While most SAM riboswitches strongly discriminate between SAM and SAH, the SAM/SAH riboswitch responds to both ligands with similar apparent affinities. The riboswitch forms an H-type pseudoknot structure with coaxial alignment of the stem–loop helix (P1) and the pseudoknot helix (PK). An additional three base pairs form at the non-open end of P1, and the ligand is bound at the interface between the P1 extension and the PK helix. Binding SAM or SAH stabilizes the PK helix, so structuring the Shine–Dalgarno sequence, sequestering it and preventing initiation of translation (OFF state).

The SAH ligand is located at the interface between the P1 and PK helices. The adenine moiety adopts an anti conformation, and the nucleobase is stacked between G46 and G24. It forms a trans Hoogsteen-Watson Crick base pair with U23 thus becoming an integral part of the coaxial P1-PK helices. The homocysteine chain is directed into the major groove of the P1 helix. The SAH adenine:U23 base pair is connected by two hydrogen bonds, i.e. adenine N6 to U23 O2 (2.9 Å) and U23 N3 to adenine N7 (2.7 Å). In addition, SAH adenine N1 accepts a hydrogen bond from U44 O2′ (2.7 Å), and the SAH O2′ donates one to G46 N7 (2.7 Å). Lastly the SAH methionyl amide N donates a hydrogen bond to U23 O4 (2.8 Å). Thus, altogether the SAH ligand forms five hydrogen bonds to the RNA that should substantially stabilize the structure of the PK helix. We observed a second molecule of SAH bound within the crystal lattice. Thus the binding site is created by the close association of the two riboswitch molecules in the crystal lattice and is unlikely to exist in free solution.

>GGUCACAACGGCUUCCUGGCGUGACCAUUGGAGCA[12x]>MFTGSIVAIVTPMDEKGNVCRASLKKLIDYHVASGTSAIVSVGTTGEFATLNHDEHADVVMMTLDLADGRIPVIAGTGANATAEAISLTQRFNDSGIVGCLTVTPYYNRPSQEGLYQHFKAIAEHTDLPQILYNVPSRTGCDLLPETVGRLAKVKNIIGIKEATGNLTRVNQIKELVSDDFVLLSGDDASALDFMQLGGHGVISVTANVAARDMAQMCKLAAEGHFAEARVINQRLMPL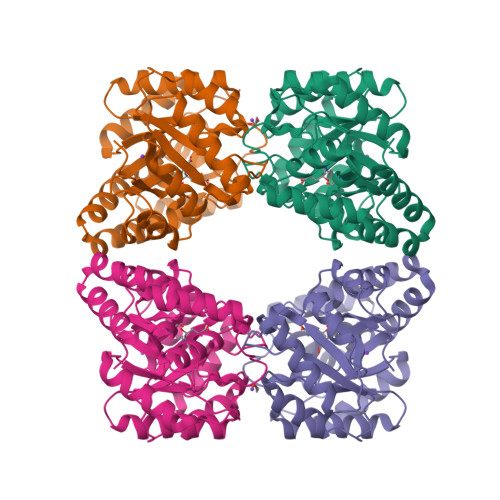HNKLFVEPNPIPVKWACKELGLVATDTLRLPMTPITDSGRETVRAALKHAGLL[2x]4-({(2S,3S)-3-[(1S)-1-(3,5-dichlorophenyl)-2-hydroxyethoxy]-2-phenylpiperidin-1-yl}methyl)-3-nitrobenzoic 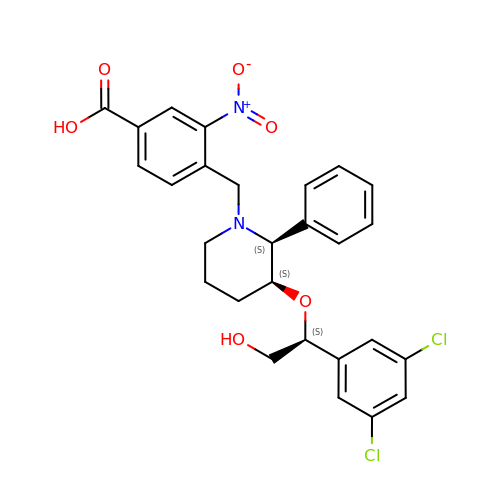acid | C27 H26 Cl2 N2 O6 | REDPQDQMPNUDEP-NXCFDTQHSA-N> MLKMFILFLISFSWYANATDFVYRVDSRPPEEIFRDGFRSHGFNRNLQQHLRGDSCAAGSRDSAFIATTTSLIETYNIARQYYSSSGFHGRLYRYRIRANNIFYPIQPSVNYLTQRGITFSGFERIMMREQNEIVAVEHIPGENIVEAVELTYDRFNSQVSDGPGTTNARYVPGSTFVNPGVIPQLVVPTVSV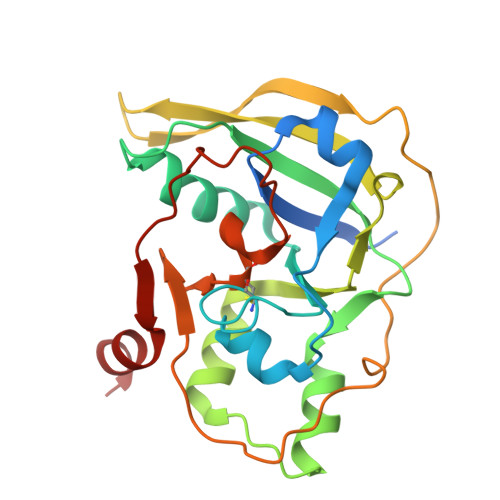RERINAFGSLISACFALKGVRRDGLNKRATYYEPEFYDARGVLKEIIK> MDQECIENYAKVNGIYIYYKLCKAPEEKAKLMTMHGGPGMSHDYLLSLRDMTKEGITVLFYDQFGCGRSEEPDQSKFTIDYGVEEAEALRSKLFGNEKVFLMGSSYGGALALAYAVKYQDHLKGLIVSGGLSSVPLTVKEMNRLIDELPAKYRDAIKKYGSSGSYENPEYQEAVNYFYHQHLLRSEDWPPEVLKSLEYAERRNVYRIMNGPNQFTITGTIKDWDITDKISAIKIPTLITVGEYDEVTPNVARVIHEKIAGSELHVFRDCSHLTMWED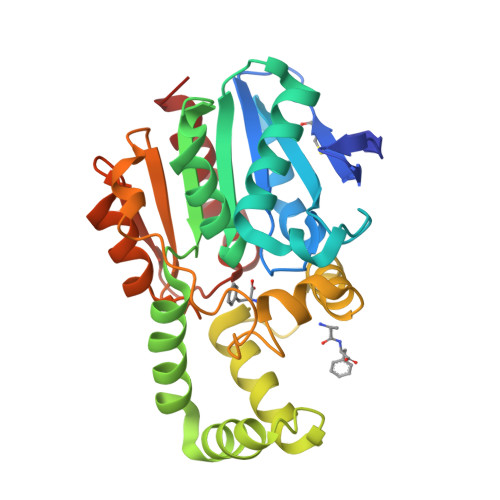REGYNKLLSDFILKHL> GIPAELRPGTNQFLTTDDDTAAPILPGFTPTPTIHIPGEVHSLLELCRVETILEVNNTTEATGLTRLLIPVSSQNKADELCAAFMVDPGRIGPWQSTLVGQICRYYTQWSGSLKVTFMFTGSFMATGKMLVAYSPPGSAQPANRETAMLGTHVIWDFGLQSSVSLVIPWISNTHFR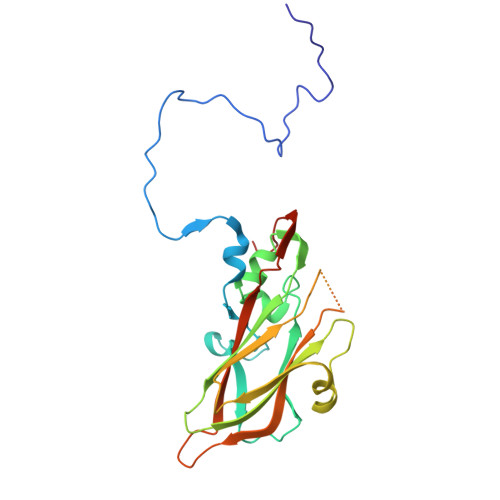TAKTGGNYDYYTAGVVTLWYQTNYVVPPETPGEAYIIAMGAAQDNFTLKICKDTDEVTQQAVLQ> MASMTGGQQMGRGSVGKTIWLQGFNNKYVNSKNGQGAMWCDSDAPQAWELFTVVDAGNGKIALRGNNGMYVSSENGEQAITCNRPAIQGWEAFDWLETADGKVSLRGSNGLFISSENGAAAMTCTRPTASGWEAFGYSVVGNA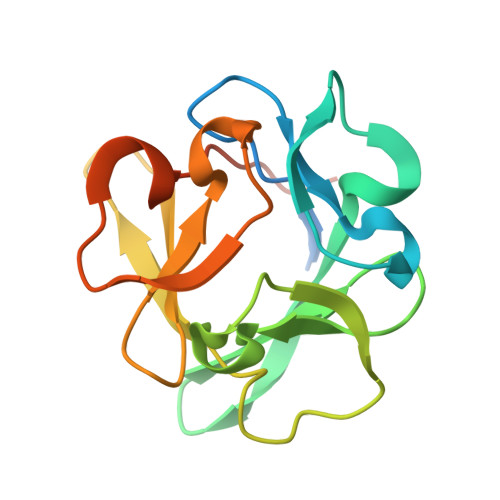LEHHHHHH One key enzyme class is the poly-β-1,6-linked N-acetyl-d-glucosamine (PNAG)-degrading glycoside hydrolases, of which the canonical member is dispersin B (DspB) from CAZy family GH20. DispTs3, DispTs2 and DispLp all consist of a single domain with the expected (β/α)8 (TIM)-barrel fold for GH20 catalytic domains. The β-strands in the centre form a tunnel atop of which the active site is located in a groove, presumably to allow long chains of PNAG to bind. GH20 enzymes use a substrate-assisted catalytic mechanism, also referred to as neighbouring-group participation (NGP), in which the reaction proceeds via the formation and subsequent breakdown of a neutral oxazoline intermediate.

A clade containing DispLp, which has 30% sequence identity to DspB along with potential dispersins from two other species, is separate from members of a second clade containing DispSf (26% sequence identity to DspB), DispTs3 (26% sequence identity to DspB) and DispTs and DispTs2 (26% and 28% sequence identity to DspB, respectively). Since DispTs3 and DispTs2 have the highest sequence identity, as expected they have a small r.m.s.d. of 0.63 Å. On the opposite side of the protein to β3, β4 and β5 is an α-helix, α7 (Lys246–Met255), in DspB and DispLp; however, this region is present as two short β-strands in DispTs3 and DispTs2. Interestingly, in the structure of unliganded DispTs3 an acetic acid solute molecule was present in a similar position to the N-acetyl group of the GlcNAc. The acetic acid also formed hydrogen bonds to Asp160 and Tyr247 with distances of 2.55 and 2.75 Å, respectively. A second tryptophan, Trp193 in DispTs3 (Trp193 in DispTs2 and Trp188 in DispLp) is present at the base of the N-acetyl group. A third tryptophan, Trp214 in DispTs3 (Trp214 in DispTs2 and Trp209 in DispLp) forms the side hydrophobic pocket in which the N-acetyl group is situated; mutation of the corresponding DspB residue, W237A, completely abolished all detectable activity on pNP-GlcNAc, suggesting that the hydrophobic pocket is essential to capture the substrate. An intense monosaccharide peak (≥5%), perhaps inferring a preferentially exo-acting enzyme, is seen for DispTs3, DispTs, DispLp and DispSf.

>[2x]QDQEKGITIDISRKYYSIKTLKAIVDEISANGGDYLQLHFSDNESYAIASEFLGQNSENPNSAYLTKKELLSLIAYSNDRNIMVIPDIDLPAHSKGWLNIMKEKDSGLYTDIVTDYSEDTLDYHNNAVALYTANQLLDEVLDLFYQPKFAGKQRIVLGGDEVPGSGAHQTDFIRFMNQIAKTAKASNYEPQMWNDSITPEGIQNLDRSFSILYWKQSTLSNGAQSLDVQDFEENGLSVYNYNAYSLYFLPSTRFTQEDITEQIDYMKWAYAYNKFFYISDYYKQVDTPNVKGSSLVFWGEHANDLSQEGLLKQEKPLIQNFLGL> SANNPWTGFQIFLSPYYANEVAAAAKQITDPTLSSKAASVANIPTFTWLDSVAKIPDLGTYLASASALGKSTGTKQLVQIVIYDLPDRDCAAKASNGEFSIANNGQANYENYIDQIVAQIQQFPDVRVVAVIEPDSLANLVTNLNVQKCANAKTTYLACVNYALTNLAKVGVYMYMDAGHAGWLGWPANLSPAAQLFTQVWQNAGKSPFIKGLATNVANYNALQAASPDPITQGNPNYDEIHYINALAPLLQQAGWDATFIVDQGRSGVQNIRQQWGDWCNIKGAGFGTRPTTNTGSQFIDSIVWVKPGGECDGTSNSSSPRYDSTCSLPDAAQPAPEAG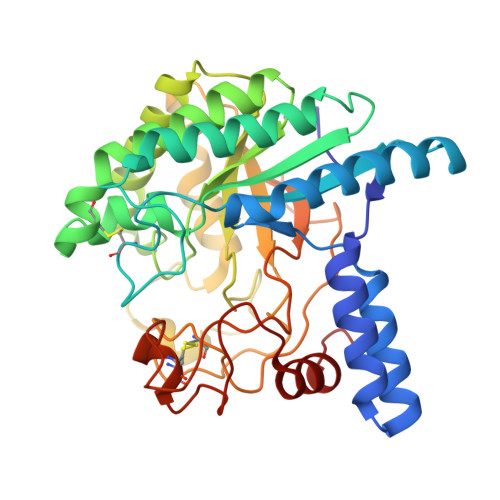TWFQAYFQTLVSAANPPL>[2x]GAHMGYQNRTLRSITSPLVAHRLKPIRQKTKKAVVSILDSEEVCVELVKEYASQEYVKEVLQISSDGNTITIYYPNGGRGFPLADRPPSPTDNISRYSFDNLPEKYWRKYQYASRFVQLVREKEPKIEYFDRYAKCILMENSPGADFEVWFYDGVKIHKTEDFIQVIEKTGKSYTLKSESEVNSLKEEIKMYMDHANEGHRICLALESIISEEERKTRSAPFFPIIIGRKPGVDSDADEEVELILGDTDSSDNSDLEDDIILSLNE

Centriole duplication begins by assembling a procentriole in the late G1/early S phase, and timely activation of Polo-like kinase 4 (Plk4) appears to be central for inducing centriole biogenesis. Plk4 dimerizes through the cryptic polo box (CPB; residues 581–808)6,8,9 of its C-terminal domain (CTD; residues 581–970) and its N-terminal kinase domain (KD)-dependent trans-autophosphorylation activity generates a phosphodegron at S285 and S289 to induce SCF-βTrCP/Slimb-mediated ubiquitination and its own proteasomal degradation. Here we demonstrate that Plk4 promotes its own ring-to-dot localization conversion by autophosphorylating and transmuting the physicochemical properties of its noncatalytic CPB, thereby causing it to rapidly coalesce into a nanoscale spherical condensate with a distinct constituent phase. Thus, we propose that Plk4 is an unparalleled kinase that harnesses its KD-dependent autophosphorylation activity to trigger its CPB-dependent physicochemical condensation.

A serendipitously generated CPB CP_v1 mutant containing a C-terminal random 32-mer extension also interacted with ANS in a similar fashion. To gain insight into how the CP mutations alter the physicochemical properties of CPB, we determined the crystal structures of both CPB CP and CPB CP_v1. While extensive efforts to obtain a high-resolution CPB CP structure yielded only a 3.7 Å overall resolution, the structure of CPB CP_v1 was solved at 2.64 Å. No densities for the C-terminal 32-mer extension of CPB CP_v1 were detected. An individual alignment of PB1 or PB2 of the CPB CP_v1 structure with the respective domain of CPB CP showed a Cα root-mean-square deviation value equal to 0.6970 or 0.7679 Å, respectively, well within the acceptable range of two superimposable structure models. Remarkably, CPB CP_v1 exhibited a substantially reduced level of twisting (119°), thus forming a greatly flattened PB2–PB2 axis. Since twisting of the β-sheet occurs as a cumulative outcome of an inherent property of the peptide backbone in each strand, the CP mutations near the PB2 base might have generated a long-distance effect along the PB2–PB2 axis, yielding largely disordered PB2-tip residues (see below). Examination of the four CP mutant residues (S698E, S700E, T704E, and T707D) revealed that each was engaged in additional interactions not found in the apo-CPB. While E698 appeared to reinforce its interaction with Q694, both E700 and E704 were involved in rigidifying the CPB CP structure by forming extra intra-subunit interactions with K600 and K711, respectively. D707 seemed to stiffen the CPB architecture by engaging in two interlocking interactions—a salt bridge with intra-subunit H771 and the other H-bonding with inter-subunit A796—thus securing the PB2 β7–β8 of one subunit to the CPB α2 backbone of the other subunit.> GPGSELPQMVQQLNSPDQQELQSALRKLSQIASGGNEQIQAVIDAGALPALVQLLSSPNEQILQEALWTLGNIASGGNEQIQAVIDAGALPALVQLLSSPNEQILQEALWTLGNIASGGNEQIQAVIDAGALPALVQLLSSPNEQILQEALWTLGNIASGGNEQIQAVIDAGALPALVQLLSSPNEQILQEALWTLGNIASGGNEQIQAVIDAGALPALVQLLSSPNEQILQEALWTLGNIASGGNEQIQAVIDAGALPALVQLLSSPNEQILQEALWTLGN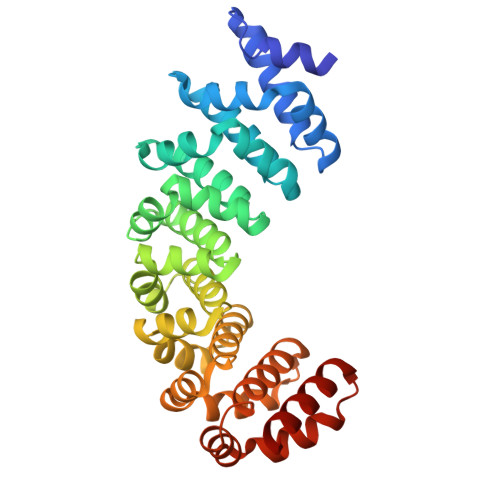IASGGNEQKQAVKEAGALEKLEQLQSHENEKIQKEAQEALEKLQSH> GHMIMANWQSIDELQDIASDLPRFIHALDELSRRLGLNITPLTADHISLRCHQNATAERWRRGFEQCGELLSENMINGRPICLFKLHEPVQVAHWQFSIVELPWPGEKRYPHEGWEHIEIVLPGDPETLNARALALLSDEGLSLPGISVKTSSPKGEHERLPNPTLAVTDGKTTIKFHP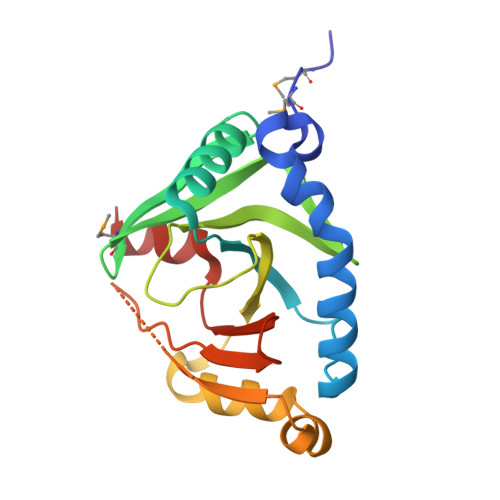WSIEEIVASEQSA2-[2-(6-oxidanylidene-1~{H}-purin-9-yl)ethyl-(4-phosphonobutyl)amino]ethylphosphonic acid | C13 H23 N5 O7 P2 | 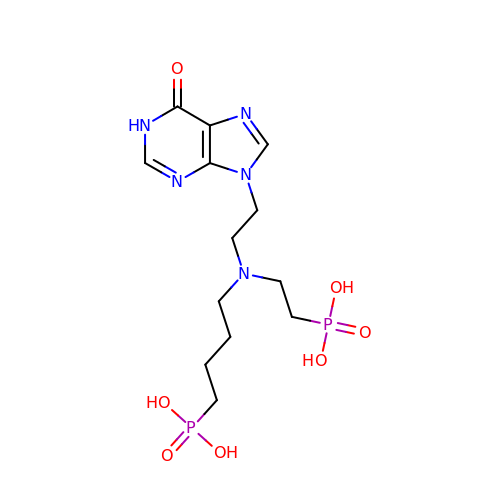UBBYDRJNNDXCEB-UHFFFAOYSA-N> GLFDKLKSLVSDDKKDTGTIEIIAPLSGEIVNIEDVPDVVFAEKIVGDGIAIKPTGNKMVAPVDGTIG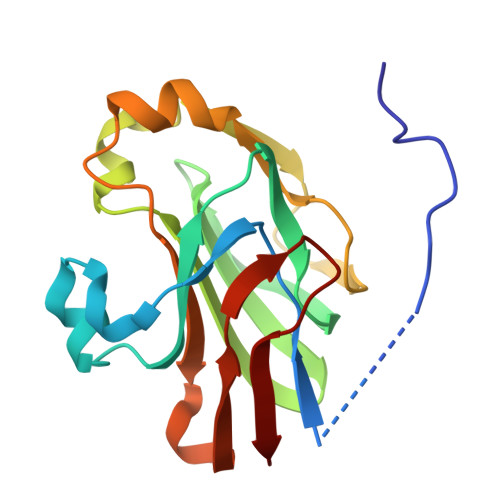KIFETNHAFSIESDSGVELFVHFGIDTVELKGEGFKRIAEEGQRVKVGDTVIEFDLPLLEEKAKSTLTPVVISNMDEIKELIKLSGSVTVGETPVIRIKK>GQDMVSPPPPIADEPLTVNTGIYLIECYSLDDKAETFKVNAFLSLSWKDRRLAFDPVRSGVRVKTYEPEAIWIPEIRFVNVENARDADVVDISVSPDGTVQYLERFSARVLSPLDFRRYPFDSQTLHIYLIVRSVDTRNIVLAVDLEKVGKNDDVFLTGWDIESFTAVVKPANFALEDRLESKLDYQLRISRQYFSYIPNIILPMLFILFISWTAFWSTSYEANVTLVVSTLIAQIAFNILVETNLPKTPYMTYTGAIIFMIYLFYFVAVIEVTVQHYLKVESQPARAASITRASRIAFPVVFLLANIILAFLFFGFGYPYDVP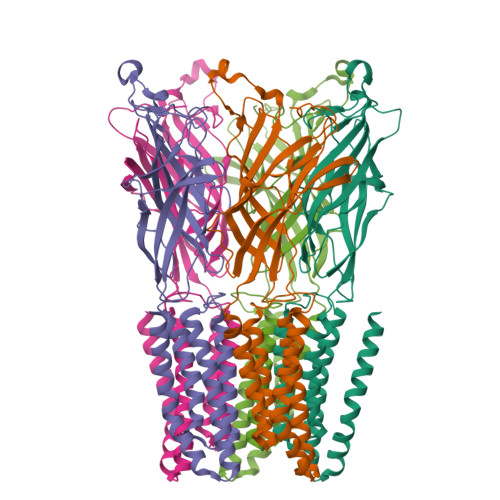DYA[5x]> AYLQDMPRSPGDVPQSPSDVSPSPDAPQSPGGMPHLPGDVLHSPGDMPHSSGDVTHSPRDIPHLPGDRPDFTQNDVQNRDMPMDISALSSPSCSPRPQSETPLEKVPWLSVMETPARKEISLSEPAKPGSAHVQSRTPQGGLYNRPCLHRLKYFLRPPVHHLFFQTLIPDKDTRENKGQRLEPIPHRRLRMVTNTIEENFPLGTVQFLMDFVSPQHYPPREIVAHIIQKILLSGSETVDVLKEAYMLLMKIQQLHPANAKTVEWDWKLLTYVMEEEGQTL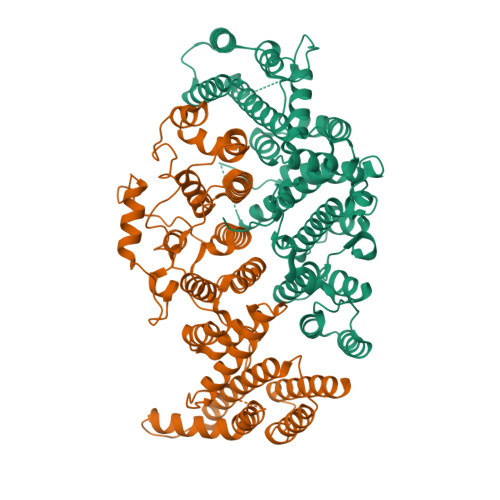PGRVLFLRYVVQTLEDDFQQTLRRQRQHLQQSIANMVLSCDKQPHNVRDVIKWLVKAVTEDGLTQPPNGNQTSSGTGILKASSSHPSSQPNLTKNTNQLIVCQLQRMLSIAVEVDRTPTCSSNKIAEMMFGFVLDIPERSQREMFFTTMESHLLRCKVLEIIFLHSCETPTRLPLSLAQALYFLNNSTSLLKCQSDKSQWQTWDELVERLQFLLSSYQHVLREHLRSSVIDRKDLIIKRIKPKPQQGDDITVVDVEKQIEAFRSRLIQMLGEPLVPQLQDKVHLLKLLLFYAADLNPDAEPFQKGWSGS;> TPAATGKPPALSKGLRSQSSDYTGHVHPGTYTNTLERLVKEMEDTQRLDELQKQLQEDIRQGRGIKSPIRIGEEDSTDDEDGLLEEHKEFLKKFSVTIDAIPDHHPGEEIFNFLNSGKIFNQYTLDLRDSGFIGQSAVEKLILKSGKTDQIFLTTQGFLTSAYHYVQCPVPVLKWLFRMMSVHTDCIVSVQILSTLMEITIRNDTFSDSPVWPWIPSLSDVAAVFFNMGIDFRSLFPLENLQPDFNEDYLVSETQTTSRGKESEDSSYKPIFSTLPETNILNVVKFLGLCTSIHPEGYQDREIMLLILMLFKMSLEKQLKQIPLVDFQSLLINLMKNIRDWNTKVPELCLGINELSSHPHNLLWLVQLVPNWTSRGRQLRQCLSLVIISKLLDEKHEDVPNASNLQVSVLHRYLVQMKPSDLLKKMVLKKKAEQPDGIIDDSLHLELEKQAYYLTYILLHLVGEVSCSHSFSSGQRKHFVLLCGALEKHVKCDIREDARLFYRTKVKDLVARIHGKWQEIIQNCRPTQGQLHDFWVPDS> MSNDNEVPGSMVIVAQGPDDQYAYEVPPIDSAAVAGNMFGDLIQREIYLQKNIYYPVRSIFEQGTKEKKEINKKVSDQVDGLLKQITQGKREATRQERVDVMSAVLHKMESDLEGYKKTFTKGPFIDYEKQSSLSIYEAWVKIWEKNSWEERKKYPFQQLVRDELERAVAYYKQDSLSEAVKVLRQELNKQKALKEKEDLSQLERDYRTRKANLQMKVQSELDQAGSALPPLVSPTPEQWLERATRLVTQAIADKKQLQTTNNTLIKNSPTPLEKQKAIYNGELLVDEIASLQARLVKLNAETTRRRTEAERKAAEEQALQDAIKFTADFYKEVTEKFGARTSEMARQLAEGARGKNIRSSAEAIKSFEKHKDALNKKLSLKDRQAIAKAFDSLDKQMMAKSLEKFSKGFGVVGKAIDAASLYQEFKISTETGDWKPFFVKIETLAAGAAASWLVGIAFATATATPIGILGFALVMAVTGAMIDEDLLEKANNLVISILEHHHHHH

Pyocin S5 (PyoS5) is a potent protein bacteriocin that eradicates the human pathogen Pseudomonas aeruginosa in animal infection models, but its import mechanism is poorly understood. In addition to its C-terminal pore-forming domain, elongated PyoS5 comprises two novel tandemly repeated kinked 3-helix bundle domains that structure-based alignments identify as key import domains in other pyocins. The central domain binds the lipid-bound common polysaccharide antigen, allowing the pyocin to accumulate on the cell surface. The N-terminal domain binds the ferric pyochelin transporter FptA while its associated disordered region binds the inner membrane protein TonB1, which together drive import of the bacteriocin across the outer membrane.

The protein crystallized in the P21 space group, and the structure was solved by a combination of single-wavelength anomalous diffraction and molecular replacement to a resolution of 2.2 Å. The first 39 residues were absent from the final model and presumed to be unstructured; we refer to this below as the “disordered region. Otherwise, continuous electron density was observed for the entirety of the remaining protein sequence (residues 40 to 498). The structure shows that PyoS5 is an elongated, α-helical protein measuring 36 Å on the short axis and 195 Å on the long axis. PyoS5 contains 17 helices, the high preponderance of helical structure likely reflecting the need to forcibly unfold the toxin during transport into a cell and the lower forces known to be required for unfolding helices relative to β-sheets. The C-terminal domain (domain 3, residues 315 to 498) has the canonical 10-helix bundle fold of a pore-forming domain found in colicins, which is consistent with the killing activity of PyoS5 (12). Domain 1 comprises residues 40 to 194, while domain 2 comprises residues 195 to 315. The core structural motif of each domain is a kinked three-helix bundle (kTHB). The other striking feature of the kTHB structural motif is that the third helix from each domain extends into the next domain of the pyocin; helix III of domain 1 extends over 90 Å into domain 2, where it forms helix I, while helix III of domain 2 extends over 90 Å to the pore-forming domain of the toxin. Moreover, over half of the 45 identical residues shared between pyocins S2, SD3, and S5 form a grooved surface that runs perpendicular to the long axis of PyoS5.> KSPLTYAEALANTIMNTYTVEELPPANRWHYHQGVFLCGVLRLWEATGEKRYFEYAKAYADLLIDDNGNLLFRRDELDAIQAGLILFPLYEQTKDERYVKAAKRLRSLYGTLNRTSEGGFWHKDGYPYQMWLNGLYMGGPFALKYANLKQETELFDQVVLQESLMRKHTKDAKTGLFYHAWDEAKKMPWANEETGCSPEFWARSIGWYVMSLADM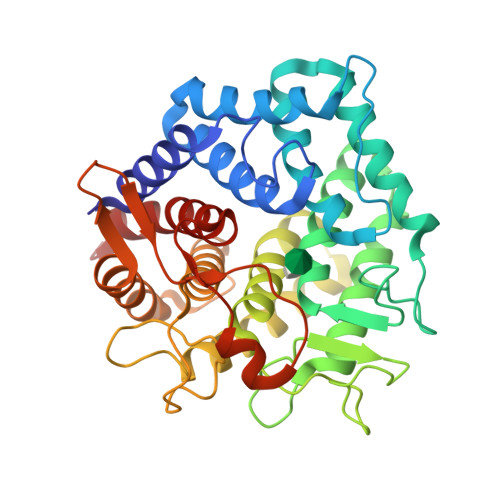IEELPKKHPNRHVWKNTLQDMIKSICRYQDKETGLWYQIVDKGDRSDNWLESSGSCLYMYAIAKGINKGYLDRAYETTLLKAYQGLIQHKTETSEDGAFLVKDICVGTSAGFYDYYVSRERSTNDLHGAGAFILAMTELEPLFRSAGK> GAMGGAHKVRAGGPGLERAEAGVPAEFSIWTREAGAGGLAIAVEGPSKAEISFEDRKDGSCGVAYVVQEPGDYEVSVKFNEEHIPDSPFVVPVASP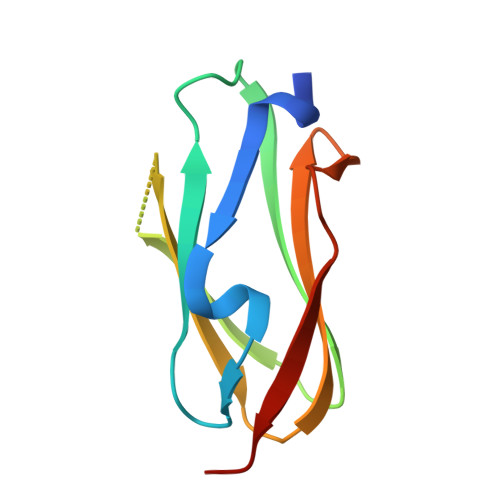S>[4x]MGHQNAAVSENQNHDDGAASSPGFKLVGFSKFVRKNPKSDKFKVKRFHHIEFWCGDATNVARRFSWGLGMRFSAKSDLSTGNMVHASYLLTSGDLRFLFTAPYSPSLSAGEIKPTTTASIPSFDHGSCR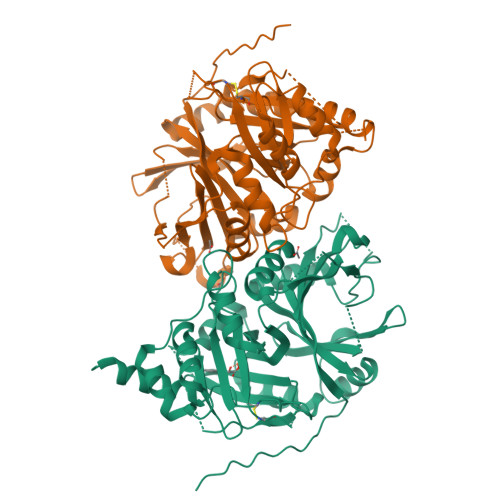SFFSSHGLGVRAVAIEVEDAESAFSISVANGAIPSSPPIVLNEAVTIAEVKLYGDVVLRYVSYKAEDTEKSEFLPGFERVEDASSFPLDYGIRRLDHAVGNVPELGPALTYVAGFTGFHQFAEFTADDVGTAESGLNSAVLASNDEMVLLPINEPVHGTKRKSQIQTYLEHNEGAGLQHLALMSEDIFRTLREMRKRSSIGGFDFMPSPPPTYYQNLKKRVGDVLSDDQIKECEELGILVDRDDQGTLLQIFTKPLGDRPTIFIEIIQRVGCMMKDEEGKAYQSGGCGGFGKGNFSELFKSIEEYEKTLEAKQLVG>GFITALPGMASVFLLMTIIFYIGAVIATKLFAASFPDWFGDLGLSAYTLFQIMTLDDWSDGIVRPVMQVYPYAWLFFVPFIMITTFAVVNLLVGLIVNSMQDAHHAEDGERTDAYRDEVLARLEQIDQR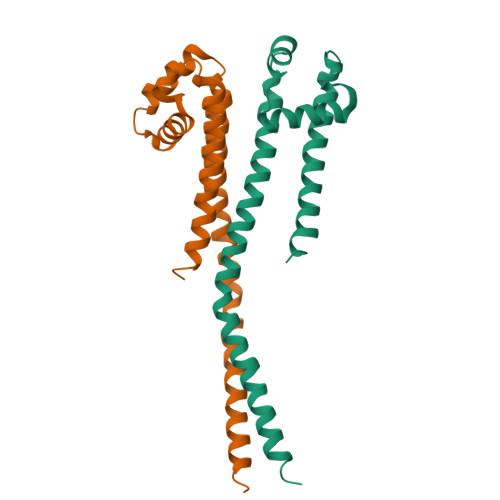LNALGETKK[2x]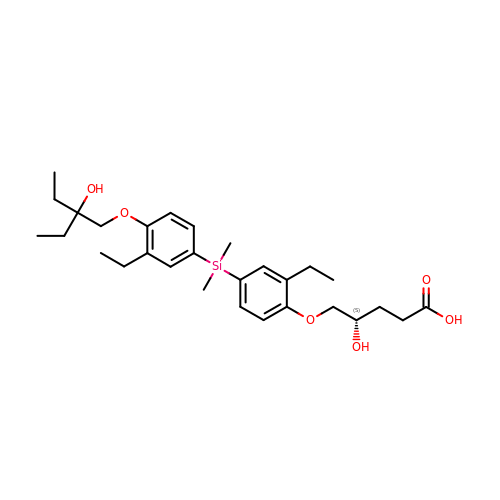(4~{S})-5-[2-ethyl-4-[[3-ethyl-4-(2-ethyl-2-oxidanyl-butoxy)phenyl]-dimethyl-silyl]phenoxy]-4-oxidanyl-pentanoic acid | C29 H44 O6 Si | GKOWYUYIKZRUDT-QHCPKHFHSA-N6-[(3S,4S)-1-benzyl-4-methylpyrrolidin-3-yl]-1-(1-methylethyl)-1,5-dihydro-4H-pyrazolo[3,4-d]pyrimidin-4-one 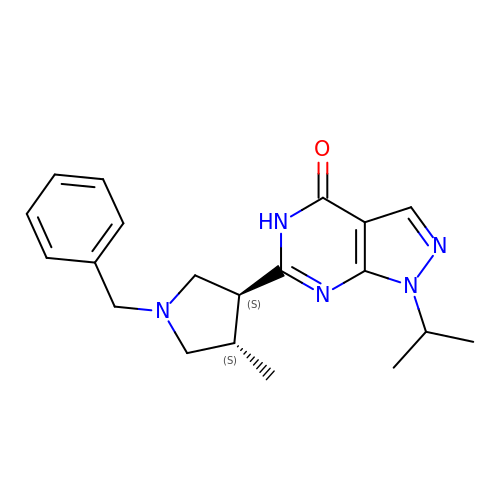| C20 H25 N5 O | PUGMRQMXTZPAIZ-RHSMWYFYSA-N3-hydroxy-7,7-dimethyl-2-phenyl-4-(thiophen-2-yl)-2,6,7,8-tetrahydro-5H-pyrazolo[3,4-b]quinolin-5-one | 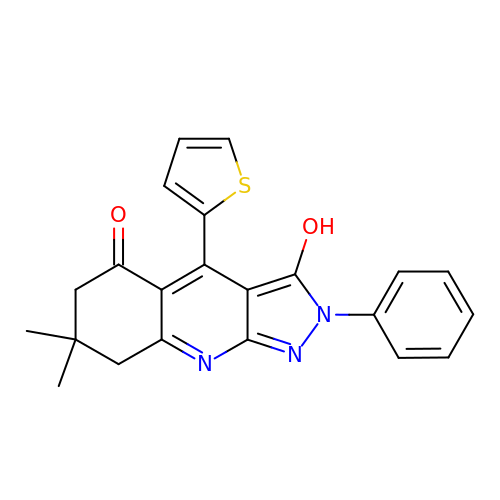C22 H19 N3 O2 S | UAVKPYTVCWRHPL-UHFFFAOYSA-N> GPHMATGQDRVVALVDMDCFFVQVEQRQNPHLRNKPCAVVQYKSWKGGGIIAVSYEARAFGVTRSMWADDAKKLCPDLLLAQVRESRGKANLTKYREASVEVMEIMSRFAVIERASIDEAYVDLTSAVQERLQKLQGQPISADLLPSTYIEGLPQGPTTAEETVQKEGMRKQGLFQWLDSLQIDNLTSPDLQLTVGAVIVEEMRAAIERETGFQCSAGISHNKVLAKLACGLNKPNRQTLVSHGSVPQLFSQMPIRKIRSLGGKLGASVIEILGIEYMGELTQFTESQLQSHFGEKNGSWLYAMCRGIEHDPVKPRQLPKTIGCSKNFPGKTALATREQVQWWLLQLAQELEERLTKDRNDNDRVATQLVVSIRVQGDKRLSSL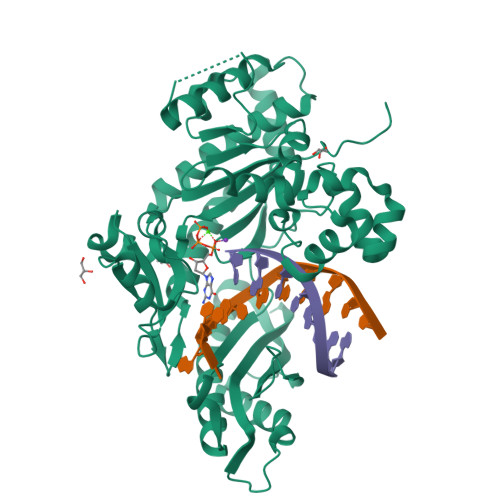RRCCALTRYDAHKMSHDAFTVIKNCNTSGIQTEWSPPLTMLFLCATKFSAS The most predominant and clinically important multidrug efflux system in C. jejuni is the CmeABC (Campylobacter multidrug efflux) pump, a tripartite system that includes an inner membrane transporter (CmeB), a periplasmic fusion protein (CmeA), and an outer membrane channel protein (CmeC). A recently identified CmeB variant, termed resistance enhancing CmeB (RE-CmeB), can increase its multidrug efflux pump activity, likely by influencing antimicrobial recognition and extrusion. The cryo-EM images of RE-CmeB without a bound ligand permitted us to resolve the structure of apo-RE-CmeB at a nominal resolution of 3.08 Å. This multidrug efflux pump adopts the overall architecture of RND-type proteins and forms a homotrimer. Each protomer is folded into a transmembrane domain containing 12 transmembrane helices (TM1 to TM12) and a periplasmic domain that can be divided into six subdomains (PN1, PN2, PC1, PC2, DN, and DC).

We reconstituted purified RE-CmeB into lipidic nanodiscs and collected single-particle images of this pump using cryo-electron microscopy (cryo-EM). The extensive classification of the single-particle images indicated that two distinct populations of RE-CmeB coexisted in this nanodisc sample. One of these structures depicted that the trimeric RE-CmeB pump does not contain any bound ligands. Interestingly, the cryo-EM structure of RE-CmeB depicts that this multidrug efflux pump forms an asymmetric trimer in which the three protomers display distinct conformational states. Similar to the structures of asymmetric AcrB, MtrDCR103 (30, 31), AdeB, and AdeJ, the three RE-CmeB protomers in our cryo-EM structure present the “access”, “binding”, and “extrusion” conformations, respectively. The entrance of the periplasmic cleft of RE-CmeB is encompassed by the amino acids Y658, L660, R710, and D823. A flexible F-loop (663PPIPGLSL670) is observed to connect the periplasmic entrance and the proximal multidrug-binding sites of RE-CmeB. A similar hydrophobic patch is found in RE-CmeB, and this RE-CmeB hydrophobic patch is composed of I178, L607, and F610. The superimposition of the apo-RE-CmeB and RE-CmeB-Amp structures shows that these two trimers are similar, with an overall root-mean-square-deviation (RMSD) of 0.6 Å.

>[3x]MFSKFFIERPIFASVVAIIISIAGIIGLANLPVEQYPSLTPPTVQVSATYTGADAQTIASTVATPIEDAINGVDNMIYMDSTSSPGQMKLTVYFNIGTDPDQAAIDVNNRISAATAKLPEAVKKLGVTVRKSSSTILEVVSVYSEDSSMNDIDIYNYVSLNILDELKRIPGVGDASAIGNKNYSMRIWLEPDLLNKFGVTANDVINAVNDQNAQYATGKIGEEPVVNKSPQVISITMQGRLQTPQEFENIILRVNEDKSFLRIKDVAKVEIGAEQYNSTGRLNTSAAVPIIINLQSGANAVNTAKLINEKMQELSKNFPQGLKYQIPYDTTIFVKASIKEVIKTFVEALALVLVVMYLFLKNFKSTIIPMIAVPVSLLGTFAVLYVLGFSINLLTLFALVLAIGIVVDDAIIVVENIDRILHEDSNISVKDAAIKAMNEVSSPVISIVLVLCAVFIPVSFISGFVGEIQRQFALTLAISVAISGFVALTLTPSLSALFLTRNESKPFYFIQKFNDFFDWSTSVFSSGVAYILKRTIRFVLVFCIMIGFIAYLFKIVPSSLVPSEDQGVIMSIINLPSGSSIHRTIEEVDTINKNATQMKEISSSVSLIGFDLFTSSLKENAAAVFFILKDWSQREASSDQIIAQLFGQYAADRNALSYFLNLPPIPGLSLTGGFEMYAQNKSGKDYDAIQQDVNKMLELARTRKELANVRTTLDTSFPQYKLIIDRDKMKYYNLNMQDVFNTISATIGTYYVNDFPMLGKNFQVNIRALGDFRNTQDALKNIYIRSSDNKMIPLNSFLTLVRSAGPDDVKRFNLFPAALIQGDPAPGYTSGQAIDAIAEVAKQSLGDEYSIAWSGSAYQEVSSKGAGAYAFVLGMIFVFLILAAQYERWLMPLAVITAVPFAVFGSILLVALRGFDNDIYFQTGLLLLIGLSAKNAILIIEFAMEERLKKGKSIFEAAINAAKLRFRPIIMTSLAFTFGVLPMIFATGAGSASRHSLGTGLIGGMIAASTLAIFFVPLFFYLLENFNEWLDKKRGKVHE> ST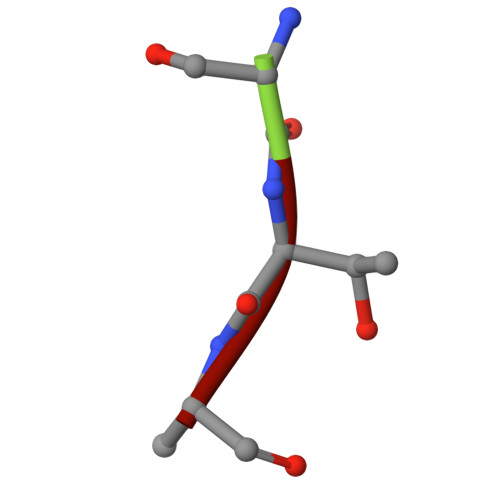A>GGKKFILELIETVYEEILDLEANLRNGQQTDSTAMWEALHIDDSSYDVNPFISMLSFDKGIKIMPRIFNFLDKQQKLKILQKIFNELSHLQIIILSSYKTTPKPTLTQLKKVDLFQMIILKIIVSFLSNNSNFIEIMGLLLQLIRNNNVSFLTTSKIGLNLITILISRAALIKQDSSRSNILSSPEISTWNEIYDKLFTSLESKIQLIFPPREYNDHIMRLQNDKFMDEAYIWQFLASLALSGKLNHQRIIIDEVRDEIFATINEAETLQKKEKELSVLPQRSQELDTE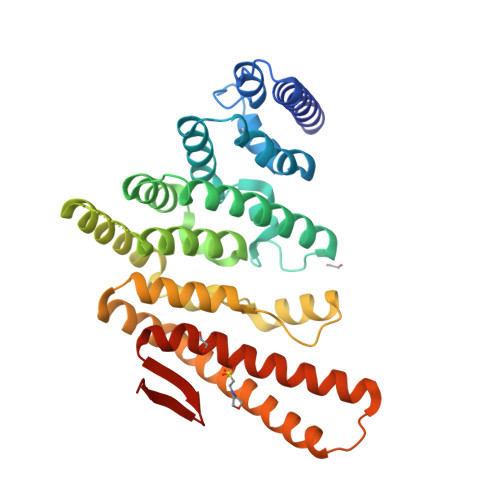LKSIIYNKEKLYQDLNLFLNVMGLVYRDGEISELKHHHHHH[2x]> GHMLFGVKCHNTDSEPLKNEDLLKNLLTMGVDIDMARKRQPGVFHRMITNEQDLKMFLLSKGASKEVIASIISRYPRAITRTPENLSKRWDLWRKIVTSDLEIVNILERSPESFFRSNNNLNLENNIKFLYSVGLTRKCLCRLLTNAPRTFSNSLDLNKQMVEFLQAAGLSLGHNDPADFVRKIIFKNPFILIQSTKRVKANIEFLRSTFNLNSEELLVLICGPGAEILDLSNDYARRSYANIKEK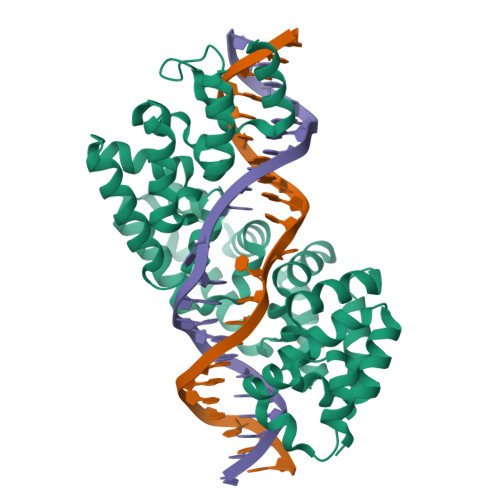LFSLGCTEEEVQKFVLSYPDVIFLAEKKFNDKIDCLMEENISISQIIENPRVLDSSISTLKSRIKELVNAGCNLSTLNITLLSWSKKRYEAKLKKLS N-{5-[(2,4-dioxo-3,4-dihydropyrimidin-1(2H)-yl)methoxy]-2-methylpentan-2-yl}benzenesulfonamide | C17 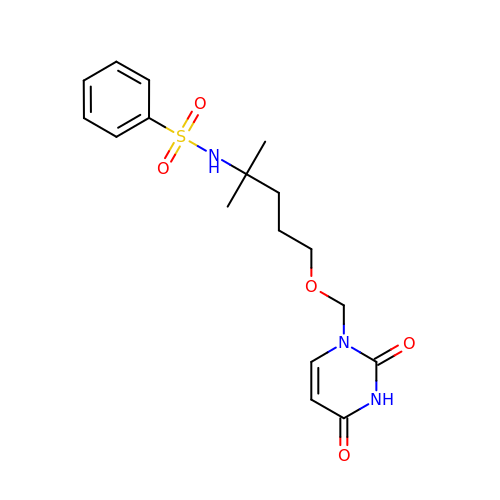H23 N3 O5 S | RMYLCQFHDYJCJN-UHFFFAOYSA-N> IHEGILFCIELSETMFKESSDLEYKSPLLEILESLDELMSQLVITRPGTAIGCYFYYCNREDAKEGIYELFPLRDINATFMKKLNDLLEDLSSGRISLYDYFMFQQTGSEKQVRLSVLFTFMLDTFLEEIPGQKQLSNKRVFLFTDIDKPQEAQDIDERARLRRLTIDLFDNKVNFATFFIGYADKPFDNEFYSDILQLGSHTNENTGLDSEFDGPSTKPIDAKYIKSRILRKKEVKRIMFQCPLILDEKTNFIVGVKGYTMYTHEKAGVRYKLVYEHEDIRQEAYSKRKFLNPITGEDVTGKTVKVYPYGDLDINLSDSQDQIVMEAYTQKDAFLKIIGFRSSSKSIHYFNNIDKSS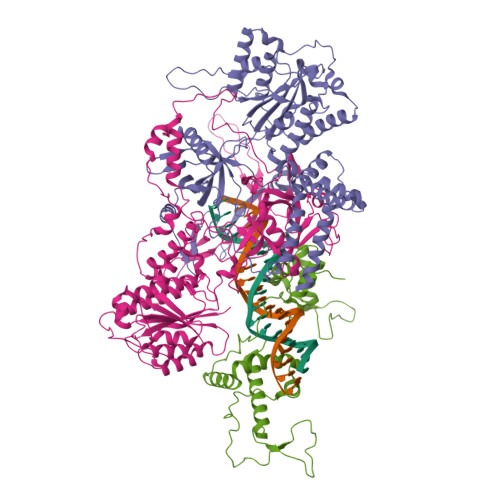FIVPDEAKYEGSIRTLASLLKILRKKDKIAILWGKLKSNSHPSLYTLSPSSVKDYNEGFYLYRVPFLDEIRKFPSLLSYDDGSEHKLDYDNMKKVTQSIMGYFNLRDGYNPSDFKNPLLQKHYKVLHDYLLQIETTFDENETPNTKKDRMMREDDSLRKLYYIRNKILESEKSEDPIIQRLNKYVKIWNMFYKKFNDDN;> SSESTTFIVDVSPSMMKNNNVSKSMAYLEYTLLNKSKKSRKTDWISCYLANCPVSENSQEIPNVFQIQSFLAPVTTTATIGFIKRLKQYCDQHSHDSSNEGLQSMIQCLLVVSLDIKQQFQARKILKQIVVFTDNLDDLDITDEEIDLLTEELSTRIILIDCGKDTQEERKKSNWLKLVEAIPNSRIYNMNELLVEITSPATSVVKPVRVFSGELRLGADILSTQTSNPSGSMQDENCLCIKVEAFPATKAVSGLNRKTAVEVEDSQKKERYVGVKSIIEYEIHNEGNKKNVSEDDQSGSSYIPVTISKDSVTKAYRYGADYVVLPSVLVDQTVYESFPGLDLRGFLNREALPRYFLTSESSFITADTRLGCQSDLMAFSALVDVMLENRKIAVARYVSKKDSEVNMCALCPVLIEHSNINSEKKFVKSLTLCRLPFAEDERVTDFPKLLDRTTTSGVPLKKETDGHQIDELMEQFVDSMDTDELPEIPLGNYYQPIGEVTTDTTLPLPSLNKDQEENKKDPLRIPTVFVYRQQQVLLEWIHQLMINDSREFEIPELPDSLKNKISPYTHKKFDSTKLVEVLGIKKV;> KASFTDEEDEFILDVVRKNPTRRTTHTLYDEISHYVPNHTGNSIRHRFRVYLSKRLEYVYEVDKFGKLVRDDDGNLIKTKVLPPSIKRKFSADEDYTLAIAVKKQFYRDLFQIDPDTGRSLITDEDTPTAIARRNMTMDPNHVPGSEPNFAAYRTQSRRGPIAREFFKHFAEEHAAHTENAWRDRFRKFLLAYGIDDYISYYEAEKAQNREPEPMKNLTNRPKRPGVPTPGNYNSAAKRARN Bacterial (1H)-3-hydroxy-4-oxoquinaldine 2,4-dioxygenase (HOD) belongs to a class of oxygenases able to catalyze this energetically unfavorable reaction without any cofactor. Arthrobacter nitroguajacolicus Rü61a (1H)-3-hydroxy-4-oxoquinaldine 2,4-dioxygenase (HOD)5 and Pseudomonas putida 33/1 (1H)-3-hydroxy-4-oxoquinoline 2,4-dioxygenase (QDO) were among the first cofactor-independent oxygenases discovered and described. They are ∼31-kDa monomeric enzymes that catalyze an O2-dependent N-heteroaromatic ring cleavage reaction with concomitant release of carbon monoxide. Remarkably, HOD and QDO are members of the α/β-hydrolase fold superfamily. The corresponding catalytic triads in HOD and QDO are Ser-101/His-251/Asp-126 and Ser-95/His-244/Asp-120, respectively.

To provide a firm structural basis to the observation that the H251A replacement essentially abolishes catalytic activity, we solved the x-ray structure of this variant in complex with the QND substrate at 1.95 Å resolution. Overall, the HOD H251A·QND complex is essentially identical to the WT HOD·QND complex solved previously under anaerobic conditions. QND binds in the catalytic pocket buried at the interface between the α/β-hydrolase fold core domain and the cap domain. The binding mode is unaffected by the H251A replacement. QND carbonyl oxygen (O4) is stabilized by a hydrogen bond (2.72 Å) with the triad's nucleophile Ser-101, whereas its NH group bonds Trp-36 carbonyl oxygen (2.75 Å). The only significant consequence of the H251A substitution is the disruption of the hydrogen bonding network connecting the QND OH group to the His-251/Asp-126 dyad. Two solvent molecules (Wat2 and Wat3 in Fig. 5B) loosely occupy the position of His-251 side chain thereby engendering an alternative network connecting QND OH group to the carboxylate group of Asp-126. However, the lack of activity for the H251A variant suggests that this water-mediated network is unable to sustain QND deprotonation. The HOD H251A·QND complex spectrum displays a peak at 341 nm with a shoulder at 354 nm. Taken together these results indicate that in the crystal as well as in solution, His-251 is responsible for the deprotonation of QND OH group.

>[4x]MRGSHHHHHHGSMDTYLHETLVFDNKLSYIDNQRDTDGPAILLLPGWCHDHRVYKYLIQELDADFRVIVPNWRGHGLSPSEVPDFGYQEQVKDALEILDQLGVETFLPVSHSHGGWVLVELLEQAGPERAPRGIIMDWLMWAPKPDFAKSLTLLKDPERWREGTHGLFDVWLDGHDEKRVRHHLLEEMADYGYDCWGRSGRVIEDAYGRNGSPMQMMANLTKTRPIRHIFSQPTEPEYEKINSDFAEQHPWFSYAKLGGPTAFPAIDVPDRAAVHIREFATAIRQGN> MEEAVLTGVATDKSEAKVTVLGISDKPGEAAKVFRALADAEINIDMVLQNVSSVEDGTTDITFTCPRSDGRRAMEILKKLQVQGNWTNVLYDDQVGKVSLVGAGMKSHPGVTA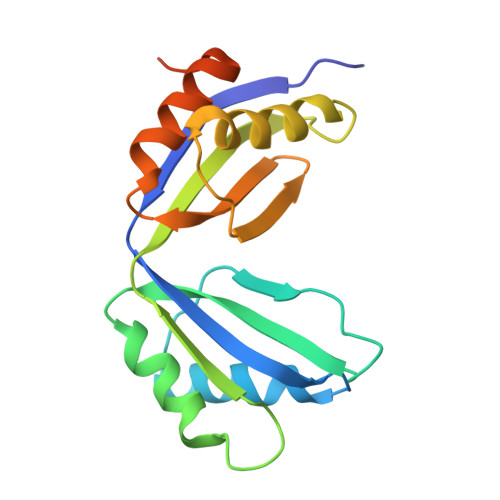EFMEALRDVNVNIELISTSEIRISVLIREDDLDAAARALHEQFQLGGEDEAVVYAGTGRHHHHHH>[4x]SMASAEKPYLKEKSSATVYFQTVKHNNIRDLVRRCITRTSQVLVILMDVFTDVEIFCDILEAANKRGVFVCVLLDQGGVKLFQEMCDKVQISDSHLKNISIRSVEGEIYC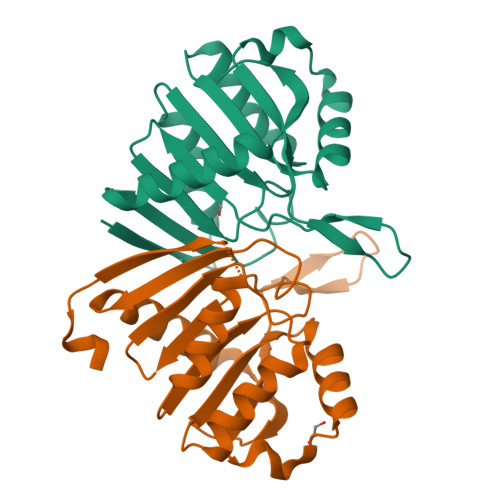AKSGRKFAGQIREKFIISDWRFVLSGSYSFTWLCGHVHRNILSKFTGQAVELFDEEFRHLYASSKPVMGLKSPRL>[4x]MNNNDIEYNAPSEIKYIDVVNTYDLEEEASKVVPHGGFNYIAGASGDEWTKRANDRAWKHKLLYPRLAQDVEAPDTSTEILGHKIKAPFIMAPIAAHGLAHATKEAGTARAVSEFGTIMSISAYSGATFEEISEGLNGGPRWFQIYMAKDDQQNRDILDEAKGDGATAIILTADSTVSGNRDRDVKNKFVFPFGMPIV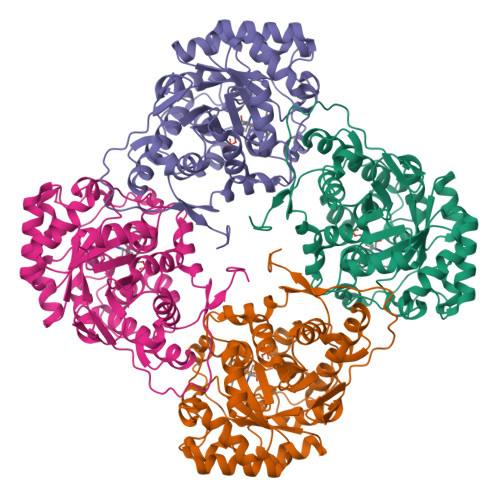QRYLRGTAEGMSLNNIYGASKQKISPRDIEEIAAHSGLPVFVKGIQHPEDADMAIKAGASGIWVSNHGARQLYEAPGSFDTLPAIAERVNKRVPIVFDSGVRRGEHVAKALASGADVVALGRPVLFGLALGGWQGAYSVLDYFQKDLTRVMQLTGSQNVEDLKGLDLFDNPYGYEY> AMKPAQKGKTFSNVEIFDPPTNYRDPQVLYARPLELSDGTLLGTWENYSPEPPNVWFPIVKSKDGGKTWKEISKVKDTQNNWGLRYQPQLYELPRAFGKYPKGTVLCSGSSIPSDLSETLIEVYASRDKGYTWEFVSHVALGGEALPNPGLTPVWEPFLMTYKEKLILYYSDQRDNATHSQKLVHQTTTDLKKWSKVVDDTKYADYYARPGMPTVAKLPNNEYIYVYEYGGGPNPPAGSDYWFPVYYRLSKDPQKFLNKAHHQIVSNDGTTPAGSPYVVWTPYGGKNGTIVVSCGTRSEIFTNQALGDASAWKKWDVPQPTAYTRSLLTFQKDPDLLMIMGAGILPPAGGKNTVSASVVRLSEV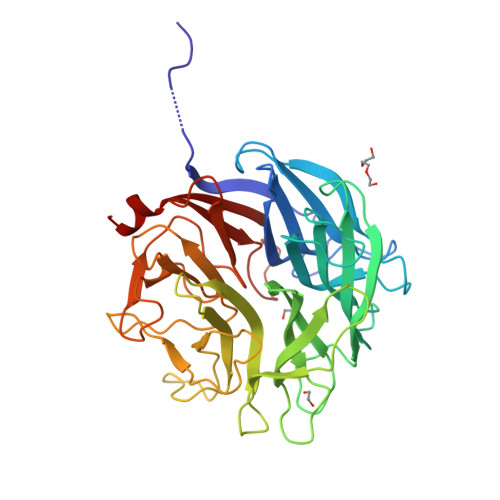MKS>[2x]MKEITFKINGQEMIVPEGTTILEAARMNNIDIPTLCYLKDINEIG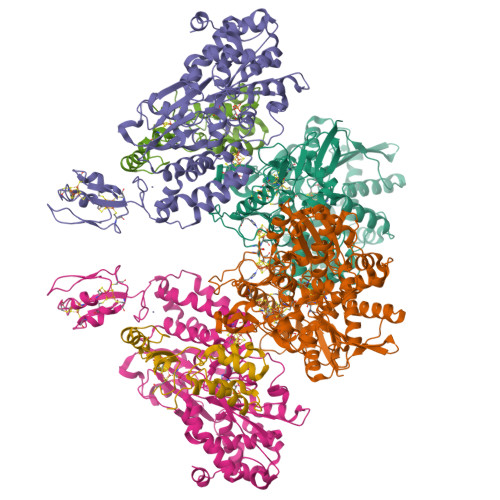ACRMCLVEIAGARALQAACVYPVANGIEVLTNSPKVREARRVNLELILSNHNRECTTCIRSENCELQTLATDLGVSDIPFEGEKSGKLIDDLSTSVVRDESKCILCKRCVSVCRDVQSVAVLGTVGRGFTSQVQPVFNKSLADVGCINCGQCIINCPVGALKEKSDIQRVWDAIADPSKTVIVQTAPAVRAALGEEFGYPMGTSVTGKMAAALRRLGFDKVFDTDFGADVCIMEEGTELIGRVTNGGVLPMITSCSPGWIKFIETYYPEAIPHLSSCKSPQNITGALLKNHYAQTNNIDPKDMVVVSIMPCTAKKYEVQREELCTDGNADVDISITTRELARMIKEARILFNKLPDEDFDDYYGESTGAAVIFGATGGVMEAAVRTVADVLNKKDIQEIDYQIVRGVDGIKKASVEVTPDLTVNLVVAHGGANIREVMEQLKAGELADTHFIELMACPGGCVNGGGQPIVSAKDKMDIDIRTERAKALYDEDANVLTYRKSHQNPSVIRLYEEYLEEPNSPKAHHILHTKYSAKPKLV;>NIDEYIGFDGYLALEKVLLTMSPVDVINEVKASGLRGRGGGGFPTGLKWQFAHDAVSEDGIKYVACNADEGDPGAFMDRSVLEGDPHAVIEAMAIAGYAVGASKGYVYVRAEYPIAVNRLQIAIDQAKEYGILGENIFETDFSFDLEIRLGAGAFVCGEETALMNSIEGKRGEPRPRPPFPANKGLFGKPTVLNNVETYANIPKIILNGAEWFASVGTEKSKGTKVFALGGKINNTGLLEIPMGTTLREIIYEIGGGIPNGKAFKAAQTGGPSGGCLPESLLDTEIDYDNLIAAGSMMGSGGLIVMDEDNCMVDVARFFLDFTQDESCGKCPPCRIGTKRMLEILERICDGKGVEGDIERLEELAVGIKSSALCGLGQTAPNPVLSTIRFFRDEYEAHIRDKKCPAGVCKHLLDFKINADTCKGCGICAKKCPADAISGEKKKPYNIDTSKCIKCGACIEACPFGSISKA[2x];>MAELIPVENLDVVKAIVAEHREVPGCLMQILQETQLKYGYLPLELQGTIADELGIPLTEVYGVATFYSQFTLKPKGKYKIGICLGTACYVRGSQAIIDKVNSVLGTQVGDTTEDGKWSVDATRCVGACGLAPVMMINEEVFGRLTVDEIPGILEKY[2x]6-HYDROXYMETHYLPTERIN 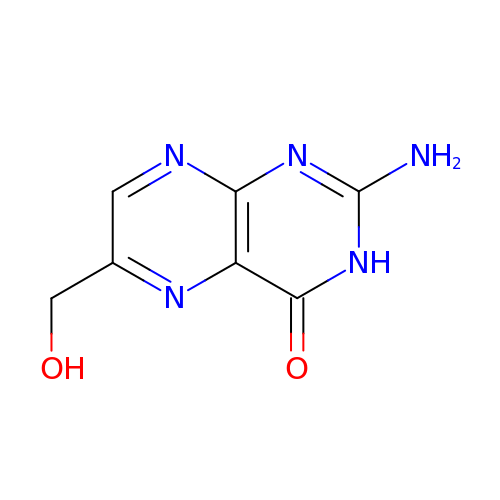| C7 H7 N5 O2 | XGWIBNWDLMIPNF-UHFFFAOYSA-N>MREKDYVVIIGSANIDVAGYSHESLNYADSNPGKIKFTPGGVGRNIAQNLALLGNKAWLLSAVGSDFYGQSLLTQTNQSGVYVDKCLIVPGENTSSYLSLLDNTGEMLVAINDMNISNAITAEYLAQHREFIQRAKVIVADCNISEEALAWILDNAANVPVFVDPVSAWKCVKVRDRLNQIHTLKPNRLEAETLSGIALSGRDDVAKVAAWFHQHGLNRLVLSMGGDGVYYSDIRGENGWSAPIKTNVINVTGAGDAMMAGLASCWVDGMPFA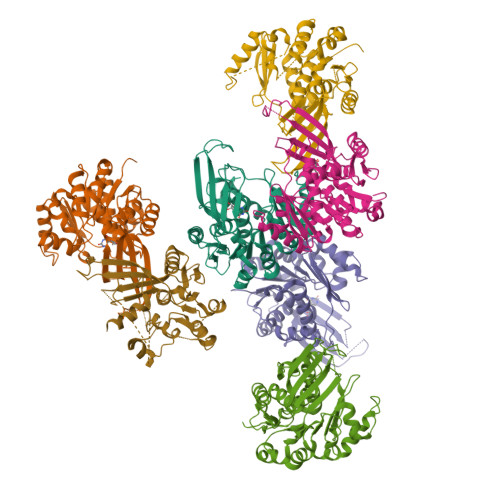ESVRFAQGCSSMALSCEYTNNPDLSIANVISLVENAECLN[8x]(2R,4S,6R)-4-amino-4,6-dimethyl-5-oxotetrahydro-2H-pyran-2-yl [(2R,3S,5R)-3-hydroxy-5-(5-methyl-2,4-dioxo-3,4-dihydropyrimidin-1(2H)-yl)tetrahydrofuran-2-yl]methyl dihydrogen diphosphate 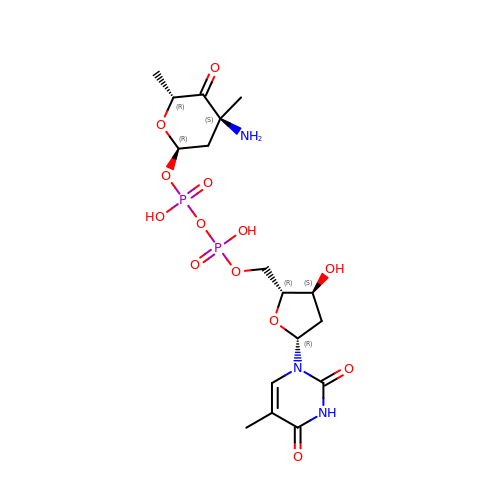(non-preferred name) | C17 H27 N3 O13 P2 | LXNLHPYBLNFMEH-XXXNSVIPSA-N> PVGAITTIEDPVLAKKVPETFPELKPGESRHTSDHMSIYKFMGRSHFLCTFTFNSNNKEYTFPITLSSTSNPPHGLPSTLRWFFNLFQLYRGPLDLTIIITGATDVDGMAWFTPVGLAVDTPWVEKESALQIDYKTA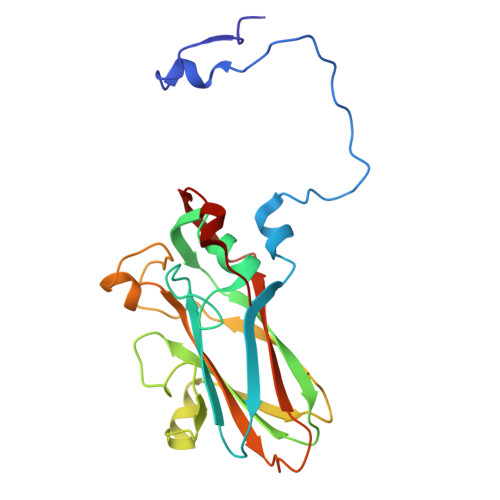LGAVRFNTRRTGNIQIRLPWYSYLYAVSGALDGLGDKTDSTFGLVSIQIANYNHSDEYLSFSCYLSVTEQSEFYFPRAPLNSNAMLST>MAEIPKEMLRAQTNVILLNVLKQGDNYVYGIIKQVKEASNGEMELNEATLYTIFKRLEKDGIIS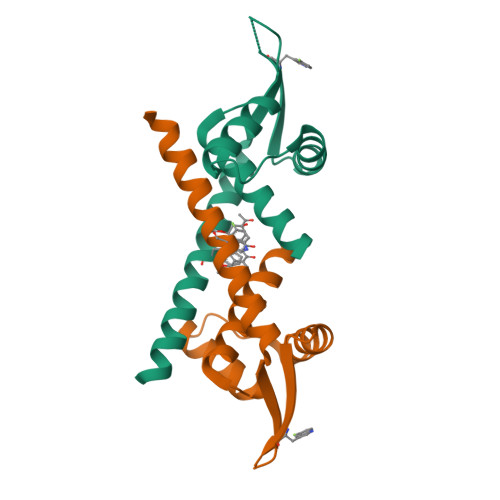SYWGDESQGGRRKYYRLTEIGHENMRLAFESWSRVDKIIENLEANKKSEAIKHHHHHH[2x]In all, we determined 23 structures, four of them not deposited in the protein data bank. These novel structures represent enzymes involved in stress response, specifically methylglyoxal reductase (YghZ), as well as three enzymes important in core metabolic functions, phosphoglucose isomerase (pGI), 6-phospho-beta-glucosidase (BglA), and glutamate dehydrogenase (GDH). All the proteins are oligomeric (YghZ, pGI, BglA, GDH) and belong to three different fold families. YghZ and BglA have a classic TIM barrel structure, pGI adopts an alpha/beta fold, and GDH possesses a core Rossmann fold found in many nucleotide binding proteins. Based on these experiments, we demonstrate successful structural characterization of multiple proteins using only microgram quantities of purified material.

The aldo-ketoreductases, of which YghZ is a member, are a large family of NADPH-dependent oxidoreductases that have the function of reducing various aldehydes and ketones. The YghZ enzyme likely functions as a methylglyoxal reductase and is known to convert the toxic metabolite methylglyoxal to acetol in vitro and in vivo. As in the larger family of aldo-keto reductases, YghZ, has a central TIM barrel domain and a smaller, mostly helical domain. YghZ is a distant homolog (<40% sequence identity) of mammalian aflatoxin dialdehyde reductases of the aldo-keto reductase AKR7 family and to potassium channel β-subunits in the AKR6 family, the structure of which was used for molecular replacement. Based on sequence alignments and structural alignments with other aldo-keto reductases, likely catalytic residues were identified in our study. Four amino acids (Tyr-66, His-138, Lys-97 and Asp-61) form a putative catalytic tetrad in the active site. Although some extra electron density was noted in the active site, the density was too diffuse to reliably model the dinucleotide cofactor or substrate/product molecules. In addition, proteins involved in stress response such as methylglyoxal reductase (YghZ) and heat shock protein 31 (HSP31) were crystallized. While these proteins are likely constitutively present at low levels under optimum growth conditions, the high cell density present during fermentor growth may lead to the induction of a stress response even when controlling for pH and aeration of the fermentor media.

>MVWLANPERYGQMQYRYCGKSGLRLPALSLGLWHNFGHVNALESQRAILRKAFDLGITHFDLANNYGPPPGSAEENFGRLLREDFAAYRDELIISTKAGYDMWPGPYGSGGSRKYLLASLDQSLKRMGLEYVDIFYSHRVDENTPMEETASALAHAVQSGKALYVGISSYSPERTQKMVELLREWKIPLLIHQPSYNLLNRWVDKSGLLDTLQNNGVGCIAFTPLAQGLLTGKYLNGIPQDSRMHREGNKVRGLTPKMLTEANLNSLRLLNEMAQQRGQSMAQMALSWLLKDDRVTSVLIGASRAEQLEENVQALNNLTFSTKELAQIDQHIADGELNLWQASSDK[8x]Although members of the tumor necrosis factor (TNF)-alpha-induced protein 8 (Tnfaip8/TIPE/Oxi-α) family were originally described as regulators of tumorigenesis, inflammation and cell death, we previously discovered novel regulatory functions for these proteins in autophagy. In particular, Tnfaip8 inhibits autophagy in an mTOR-dependent manner under oxidative stress conditions. In conclusion, our data demonstrate that mTnfaip8 is a novel phosphoglyceride binding protein with PE as the most preferred substrate. PE binding in the hydrophobic cavity allows it to form a ternary complex with Gαi3, mTnfaip8-PE-Gαi3, and to mediate insulin-induced anti-autophagy.

The crystal structure of Tnfaip8 from Mus musculus (mTnfaip8) was determined at 2.03 Å resolution. Except for 12 flexible N-terminal residues (Met1-Ala12), all other amino acids are defined in the electron density map. The overall shape of mTnfaip8 resembles a water dipper. Its cylindrical domain has a dimension of 48 Å × 31 Å × 30 Å connected to an N-terminal grip-like domain composed of 20 residues with a length of ~35 Å. The dimensions of the hydrophobic cavity are ~20 Å in depth and ~7 Å in diameter at the bottom up to ~10 Å at the entrance. The cavity is lined with highly conserved hydrophobic residues. Intriguingly, two long electron densities were found inside the cylindrical domain of mTnfaip8. hTIPE2 and hTIPE3 also contain similar densities in the cavities of their cylindrical domains. As the most promising PE candidate, PE 34:1 was selected and modeled into the cavity because the known major FA compositions of PE from E. coli are C16:0 (36%) and C18:1 (31%). The PE-bound model explained a potent functional role of the three positively charged residues, H86, R87, K103, near the entrance of the cavity. These amino acids are next to the phosphate moiety of PE.

> MLSEAEEPREVATDVFNSKNLAVQAQKKILGKMVSKSIATTLIDDTSSEVLDELYRVTKEYTQNKKEAERVIKNLIKTVIKLAVLHRNNQFNQDELALMEKFKKKVHQLAMTVVSFHQVEYTFDRNVLSRLLNECRELLHEIIQRHLTAKSHGRVNNVFDHFSDSDFLAALYNPFGKFKPHLQKLCDGINKMLDEENI>MKASPHRPTKALIHLGAIRQNIQQMGAHIPQGTLKLAVVKANAYGHGAVAVAKAIQDDVDGFCVSNIDEAIELRQAGLSKPILILGVSEIEAVALAKEYDFTLTVAGLEWIQALLDKEVDLTGLTVHLKIDSGMGRIGFREASEVEQAQDLLQQHGVCVEGIFTHFATADEESDDYFNAQLERFKTILASMKEVPELVHASNSATTLWHVETIFNAVRMGDAMYGLNPSGAVLDLPYDLIPALTLESALVHVKTVPAGACMGYGATYQADSEQVIATVPIGYADGWTRDMQNFSVLVDGQACPIVGRVSMDQITIRLPKLYPLGTKVTLIGSNGDKEITATQVATYRVTINYEVVCLLSDRIPREYY[2x]

The bacterial enzyme alanine racemase (Alr; E.C. 5.1.1.1) uses a covalently-bound pyridoxal 5"-phosphate (PLP) cofactor to catalyze the racemization of L-alanine and D-alanine, the latter being an essential component of the peptidoglycan layer in bacterial cell walls. The lack of alanine racemase function in eukaryotes makes this enzyme an attractive target for antimicrobial drug development. In all of these structures, Alr is a homodimeric enzyme formed by a head-to-tail association of two monomers. The active site in each monomer is located in the centre of the α/β barrel and contains a pyridoxal phosphate (PLP) co-factor covalently connected to a lysine residue by an internal aldimine bond.

Here we report the crystal structure of alanine racemase from S. pneumoniae (AlrSP). Crystals diffracted to a resolution of 2.0 Å and belong to the space group P3121 with the unit cell parameters a = b = 119.97 Å, c = 118.10 Å, α = β = 90° and γ = 120°. AlrSP forms a homodimer in which the two monomers form a head-to-tail association, typical of that seen in other alanine racemases. Each monomer has an eight-stranded α/β barrel domain (residues 1-238) and an extended β-strand domain (residues 239-367). The pyridoxal phosphate (PLP) cofactor is connected to Lys40 through an internal aldimine bond and resides inside the α/β barrel domain. As an incidental finding, the AlrSP structure contained additional electron density within the A monomer, at the end of helix 1 in the N-terminal α/β barrel domain. This planar density resembled a carboxylated aromatic ring, therefore a benzoic acid molecule, which fitted and refined well, was modeled into this region, even though the compound was not added to purification or crystallization conditions (topology and parameters obtained from the Hetero-compound Information Centre-Uppsala, HIC-UP). We observed electron density consistent with a carbamylated lysine at the NZ terminus of Lys129, as seen in most other alanine racemase structures. The smallest constriction in the entryway corridor of AlrSP is between Tyr263' and Tyr352 of the inner layer, which provide an opening width of only about 2.6Å for an active site inhibitor to pass through (the distance between the closest atoms of these two side chains with the van der Waals radius for each atom subtracted). A cluster of hydrogen-bonded water molecules forms an ordered pentagonal ring and some adjacent partial rings in the active site entryways of both monomers of AlrSP.>SGISLDNSYKMDYPEMGLCIIINNKNFHKSTGMTSRSGTDVDAANLRETFRNLKYEVRNKNDLTREEIVELMRDVSKEDHSKRSSFVCVLLSHGEEGIIFGTNGPVDLKKITNFFRGDRCRSLTGKPKLFIIQACRGTELDCGIETD[2x];>SGVDDDMACHKIPVEADFLYAYSTAPGYYSWRNSKDGSWFIQSLCAMLKQYADKLEFMHILTRVNRKVATEFESFSFDATFHAKKQIPCIVSMLTKELYFYH[2x];>[2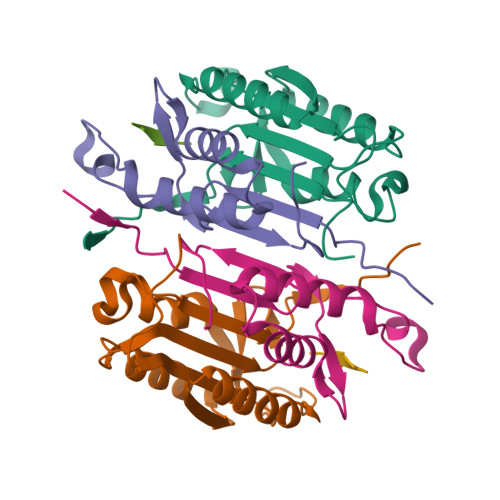x]XDVPD>[6x]MSTLSGPQYLGEGLKLMMRPGLR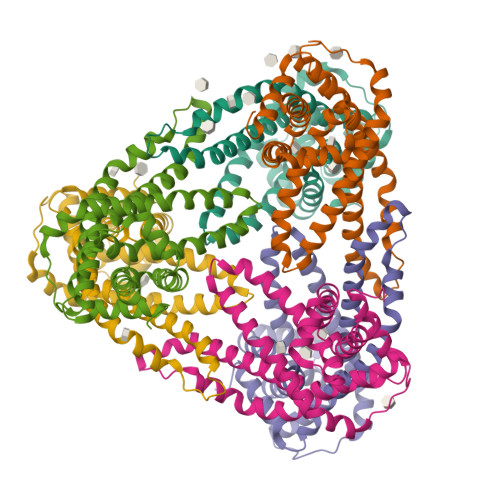LFVLLPLSINLILFIGLIGFAINQFSHWVDWLMPSLPEWLSFLQFILWPLFVTLVLLIVFFTFTLIANLIAAPFNGFLAEKVEVVVRGTDDFPAFSWAELMAMVPRTIGRELRKLGYFLPRAIALFILSLIPGLNLIAAPLWLLFGVWMMAVQYIDYPADNHKLGWNEMLAWLRSKRWACMGFGGITYLVLLIPLVNLVAMPAAVAGAVLFWVREGGDQALVK>[2x]AQRGAGAGAAEPGPPRTPRPGRREPVMPRPPVPANALGARGEAVRLQLQGEELRLQEESVRLHQINIYLSDRISLHRRLPERWNPLCKEKKYDYDNLPRTSVIIAFYNEAWSTLLRTVYSVLETSPDILLEEVILVDDYSDREHLKERLANELSGLPKVRLIRANKREGLVRARLLGASAARGDVLTFLDCHCECHEGWLEPLLQRIHEEESAVVCPVIDVIDWNTFEYLGNSGEPQIGGFDWRLVFTWHTVPERERIRMQSPVDVIRSPTMAGGLFAVSKKYFEYLGSYDTGMEVWGGENLEFSFRIWQCGGVLETHPCSHVGHVFPKQAPYSRNKALANSVRAAEVWMDEFKELYYHRNPRARLEPFGDVTERKQLRDKLQCKDFKWFLETVYPELHVPEDRPGFFGMLQNKGLTDYCFDYNPPDENQIVGHQVILYLCHGMGQNQFFEYTSQKEIRYNTHQPEGCIAVEAGMDTLIMHLCEETAPENQKFILQEDGSLFHE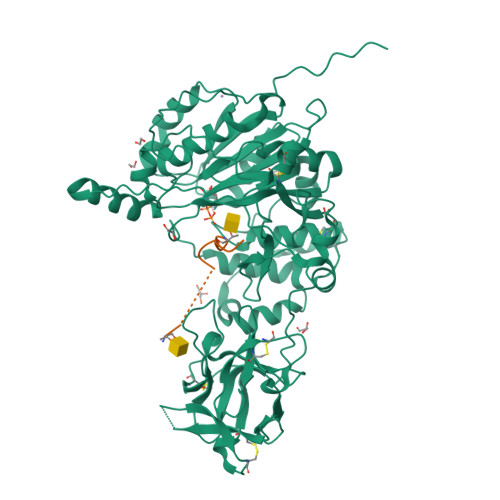QSKKCVQAARKESSDSFVPLLRDCTNSDHQKWFFKERML;>[2x]GAGATGAGAGYYITPRTGAGA>RAKGGAPGFKVAILGAAGGIGQPLAMLMKMNPLVSVLHLYDVVNAPGVTADISHMDTGAVVRGFLGQQQLEAALTGMDLIIVPAGVPRKPGMTRDDLFKINAGIVKTLCEGIAKCCPRAIVNLISNPVNSTVPIAAEVFKKAGTYDPKRLLGVTMLDVVRANTFVAEVLGLDPRDVDVPVVGGHAGVTILPLLSQVKPPSSFTQEEISYLTDRIQNGGTEVVEAKAGAGSATLSMAYAAVKFADACLRGLRGDAGVIECAFVSSQV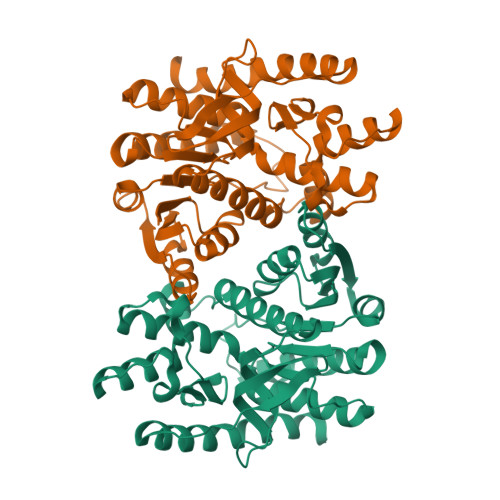TELPFFASKVRLGRNGIEEVYSLGPLNEYERIGLEKAKKELAGSIEKGVSFIRSHHHHHH[8x]>MDIVAPDRTRIAPEIDRDEALEGDRESDPALASTREWQLEDMPRWQDELTVRGLVAALLIGFIYTVIVMKIALTTGLVPTLNVSAALLSFLALRGWTRLLERFGVVSRPFTRQENTIVQTCGVACYTIAFAGGFGSTLLGLNKKTYELAGDSPGNVPGSWKEPGIGWMTGFLLACSFGGLLTLIPLRQVLVVDYKLVYPSGTATAILINGFHTDQGDKNSRKQIRGFLKYFGGSFLWSFFQWFYTGGDACGFVQFPTFGLKAWKQTFYFDFSMTYVGAGMICPHIVNISTLLGAIISWGIMWPLISKNKGDWYPAKVPESSMKSLYGYKAFICIALIMGDGMYHFIKIVGITAMSMYRQFSHKQVNNKAKNADDTVSLEELHRQEIFKRGHIPSWMAYAGYALFSVLAVVTIPVMFKQVKWYYVVIAYVVAPMLGFANSYGTGLTDINMGYNYGKIALFVFAGWAGKENGVIAGLVAGTLVKQLVLISADLMQDFKTSYLTQTSPKSMMIAQVVGTAMGCIVSPLTFMLFYKAFDIGNPDGTWKAPYALIYRNMAILGVEGFSVLPKYCIVISGGFFAFAAILSITRDVMPHKYAKYVPLPMAMAVPFLVGGSFAIDMCLGSLIVFAWTKINKKEAGFMVPAVASALICGDGIWTFPASILALAKIKPPICMKFLPAATSAAHHHHHHHH[2x]

Poaceae species use a unique chelation strategy, whereby plants secrete a high-affinity metal chelator, known as phytosiderophores (mugineic acids), and reabsorb the iron-phytosiderophore complex by the yellow stripe 1/yellow stripe 1-like (YS1/YSL) transporter for efficient uptake of iron from the soil. Here, we present three cryo-electron microscopy structures of barley YS1 (HvYS1) in the apo state, in complex with an iron-phytosiderophore complex, Fe(III)-deoxymugineic acid (Fe(III)–DMA), and in complex with the iron-bound synthetic DMA analog (Fe(III)–PDMA). The structures reveal a homodimeric assembly mediated through an anti-parallel β-sheet interaction with cholesterol hemisuccinate. HvYS1 comprises two distinct domains: a substrate-binding YS core and a scaffold domain, implicating an elevator-like transport.

To overcome these limitations of DMA, proline 2’-deoxymugineic acid (PDMA), a DMA analog, was synthesized by replacing the four-membered azetidine ring with a five-membered ring. PDMA effectively substituted DMA for iron uptake by HvYS1 in the insect-cell assay system, and significantly improved the growth of rice in calcareous soil. In order to verify if PDMA functions in YS1 in the same manner as DMA, we determined the cryo-EM structure of HvYS1 in complex with Fe(III)–PDMA to an overall resolution of 2.9 Å. The HvYS1 structure bound to Fe(III)–PDMA reveals the outward open conformation, nearly identical to the apo and the Fe(III)–DMA bound structures. Fe(III)–PDMA occupies the same binding site as Fe(III)–DMA, demonstrating that PDMA can function as a potent fertilizer in an essentially identical manner to DMA. The carboxyl and amino group moieties of PDMA are recognized by YS1 in the same manner as those of DMA. The five-membered ring of PDMA is well fit with the binding pocket for the four-membered ring without any steric clashes. Our cryo-EM data supports that PDMA activity as a potent fertilizer uses the same mechanism as DMA.Another unicellular pappalysin is the T. forsythia KLIKK MP mirolysin, which protects the bacterium against complement-mediated bactericidal activity. It is secreted as a 66 kDa zymogen (see UniProt code A0A0F7IPS1), which when activated cleaves several physiologically relevant host proteins such as fibronectin; fibrinogen; complement proteins C3, C4 and C5; as well as antimicrobial peptide LL-37. As part of its virulence factor armamentarium, at the site of colonization it secretes mirolysin, a metallopeptidase of the unicellular pappalysin family, as a zymogen that is proteolytically auto-activated extracellularly at the Ser54–Arg55 bond. The catalytic domain conforms to the metzincin clan of metallopeptidases and contains a double calcium site, which acts as a calcium switch for activity.

We next obtained a product complex of mature mirolysin with a tetradecapeptide (Lys1–Lys14) occupying S1′ and further primed sub-sites of the cleft plus a citrate in S1 (CIT−1). However, a tetradecapeptide from the lipoprotein was found covering sub-sites S1′ to S6′ and more of the primed side of the active-site cleft [for sub-site and peptide substrate nomenclature, see Schechter & Berger and Gomis-Rüth, Botelho et al.]. Moreover, a citrate anion was attached to S1 on the non-primed side. Thus, we serendipitously trapped a product complex, which revealed the molecular determinants of substrate binding and catalysis of mirolysin (see Section 3.5). Citrate CIT−1 mimics an amino acid in S1 after catalysis. The side chain of Lys1 intrudes into the S1′ specificity pocket and binds the main-chain carbonyl of Thr287 at the pocket bottom. Lys1 Nζ is linked to Asp289 Oδ1 through an internal solvent-mediated salt bridge, which explains the preference for basic residues in S1′.

> RSVPSSTILIPVVVHVVYNNSAQNISDAQIISQIQVLNEDFRRMNADQANTPSAFANLAGNANIEFKLARRDPNGNTTNGITRTSTSTETFSMEMDNVKFSNLGGNNAWNTRRYLNIWVCNLGDDLLGYAQFPFEFQTKPNTDGVVIHYKHFGRDGSAESPYDKGRTATHEVGHWLDLRHIWGDDGGSCSGTDNIADTPNQGGYNEGCPSFPKTDHCTNTSPGVMFMNYMDYTYDACMNLFTKGQVERMRSLFDTQTGIRREMQIYANELTNPLSFS;> KRDPVYFIKLSTIK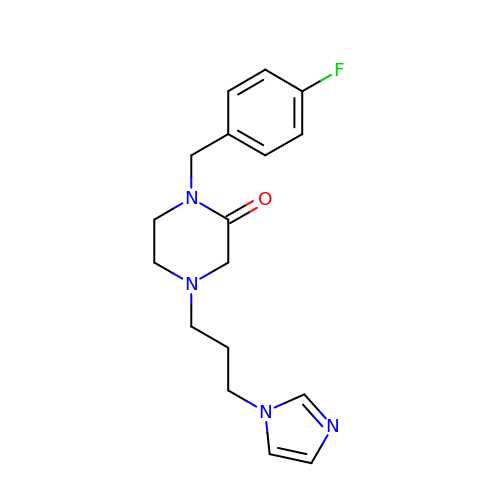1-[(4-fluorophenyl)methyl]-4-(3-imidazol-1-ylpropyl)piperazin-2-one | C17 H21 F N4 O | NBFKCPBQLPIJMN-UHFFFAOYSA-N>[2x]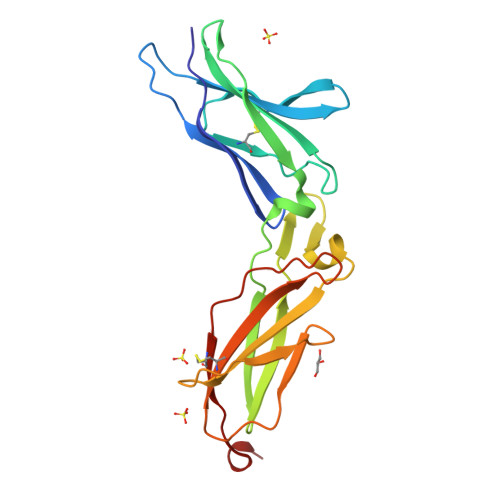MVPPPENVRMNSVNFKNILQWESPAFAKGQLTFTAQYLSYRIFQDKCMQTTLTECDFSSLSKYGDHTLRVRAEFADEHSDWVQITFSPVDDTIIGPPGMQVEVLADCLHMRFLAPKIENEYETWTMKNVYNSWTYNVQYWKQGTDEKFQITPQYDFEVLRNLEPWTTYCVQVRGFLPDRNKAGEWSEPVCEQTTHDETVPS>[2x]GRKERERLEEKLEDANERIAELVKLEERQRMARDLVDTLGQKLSLMGLKSDLARKLIYKDPEQAARELKSVQQTARTSL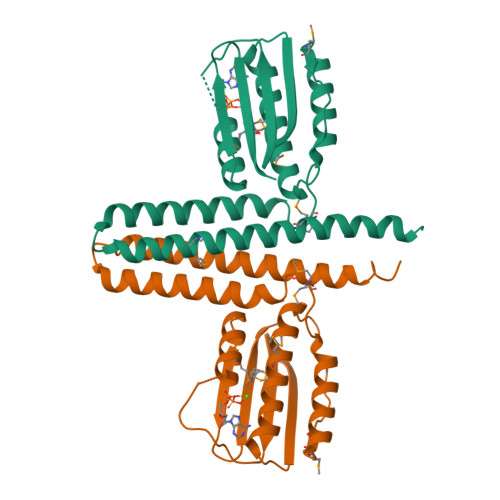NEVRKIVSSMKGIRLKDELINIKQILEAADIMFIYEEEKWPENISLLNENILSMCLKEAVTNVVKHSQAKTCRVDIQQLWKEVVITVSDDGTFKGEENSFSKGHGLLGMRERLEFANGSLHIDTENGTKLTMAIPNNSK>MARKFVVGGNWKMNGDKKQINEIIGFLKSGPLNQDTEVVVGVPAIYLELVRTCVPASIGVAAQNCYKVPKGAFTGEISPAMIKDVGADWVILGHSERRQIFGESDELIAEKVCHALESGLKVIACIGETLEEREAGKTEEVVFRQTKAIAAKVNDWSNVVIAYEPVWAIGTGKTATPQQAQDVHKALRQWICENIDAKVGNSIRIQYGGSVTAANCKELASQPDIDGFLVGGASLKPEFVDIINARQLVPRGSHHHHHH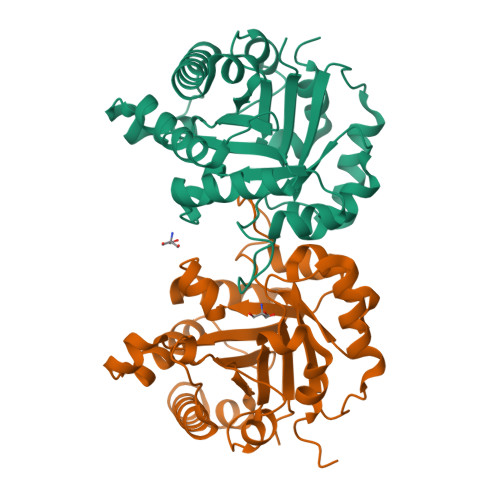[4x]4-({4-[(2-chlorophenyl)amino]-5-fluoropyrimidin-2-yl}amino)benzoic acid | C17 H12 Cl F N4 O2 | 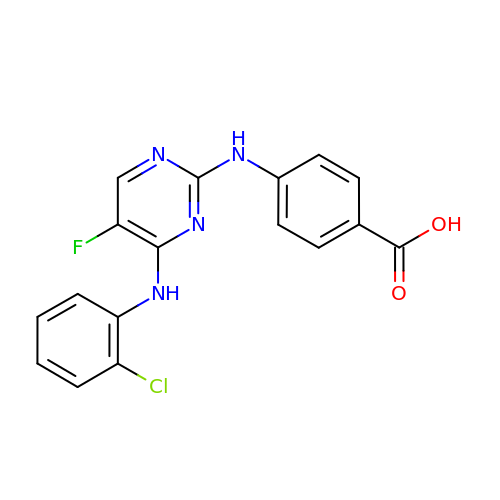BLFRZPJRKJLHGU-UHFFFAOYSA-N> GSSGSSGKDNIRHGVCWIYYPDGGSLVGEVNEDGEMTGEKIAYVYPDERTALYGKFIDGEMIEGKLATLMSTEEGRPHFELMPGNSVYHFDKSTSSCISTNALLPDPYESERVYVAESLISSAGEGLFSKVAVGPNTVMSFYNGVRITHQEVDSRDWALNGNTLSLDEETVIDVPEPYNHVSKYCASLGHKANHSFTPNCIYDMFVHPRFGPIKCIRTLRAVEADEELTVA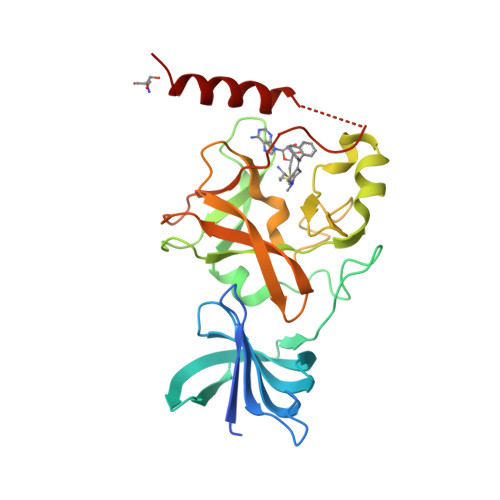YGXXXXXXXXXXXXXPEWYQVELKAFQATQQK5-hydroxynaphthalene-1,4-dione 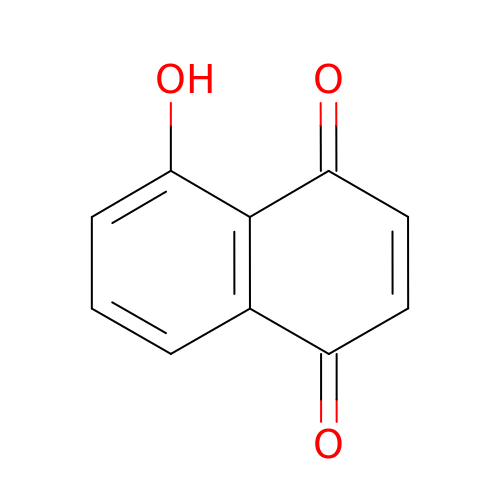| C10 H6 O3 | KQPYUDDGWXQXHS-UHFFFAOYSA-N>[2x]MGSSHHHHHHSSGLVPRGSHMSPSPVPGSQNVPAPAVKKISQYACQRRTTLNNYN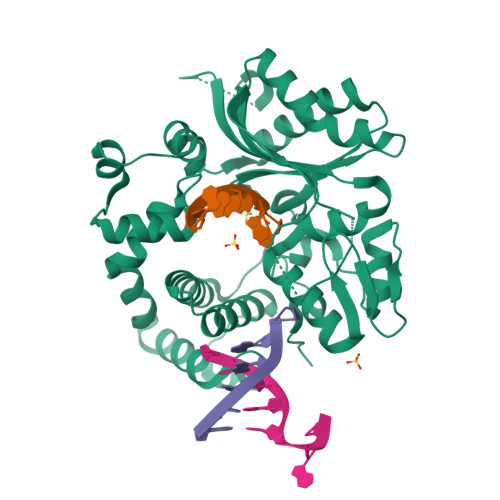QLFTDALDILAENDELRENEGSCLAFMRASSVLKSLPFPITSMKDTEGIPCLGDKVKSIIEGIIEDGESSEAKAVLNDERYKSFKLFTSVFGVGLKTAEKWFRMGFRTLSKIQSDKSLRFTQMQKAGFLYYEDLVSCVNRPEAEAVSMLVKEAVVTFLPDALVTMTGGFRRGKMTGHDVDFLITSPEATEDEEQQLLHKVTDFWKQQGLLLYCDILESTFEKFKQPSRKVDALDHFQKCFLILKLDHGRVHSEKSGQQEGKGWKAIRVDLVMCPYDRRAFALLGWTGSRQFERDLRRYATHERKMMLDNHALYDRTKRVFLEAESEEEIFAHLGLDYIEPWERNA> GTSCPVNWVEHQDSCYWFSHSGMSWAEAEKYCQLKNAHLVVINSREEQNFVQKYLGSAYTWMGLSDPEGAWKWVDGTDYATGFQNWKPGQPDD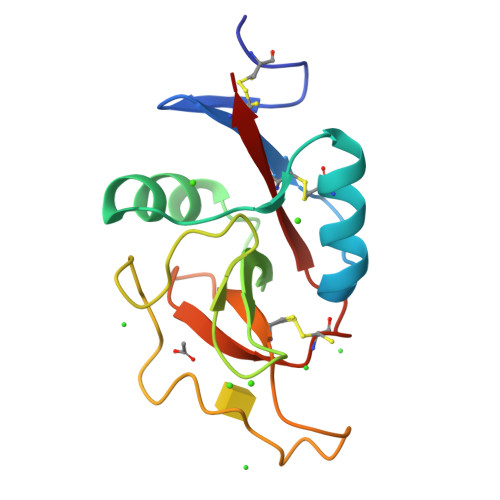WQGHGLGGGEDCAHFHPDGRWNDDVCQRPYHWVCEAGLG>[6x]MPPREVHVQVTHSMPPQKIEIFKSLDNWAEENILVHLKPVEKCWQPQDFLPDPASDGFDEQVRELRERAKEIPDDYFVVLVGDMITEEALPTYQTMLNTLDGVRDETGASPTSWAIWTRAWTAEENRHGDLLNKYLYLSGRVDMRQIEKTIQYLIGSGMDPRTENSPYLGFIYTSFQERATFISHGNTARQAK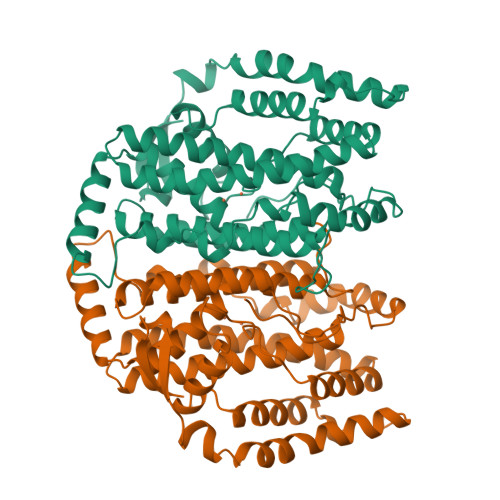EHGDIKLAQICGTIAADEKRHETAYTKIVEKLFEIDPDGTVLAFADMMRKKISMPAHLMYDGRDDNLFDHFSAVAQRLGVYTAKDYADILEFLVGRWKVDKLTGLSAEGQKAQDYVCRLPPRIRRLEERAQGRAKEAPTMPFSWIFDRQVKL2-[(2S,3R,4S,5R)-5-(aminomethyl)-3,4-dihydroxytetrahydrofuran-2-yl]-N-(pyridin-2-ylmethyl)acetamide | C13 H19 N3 O4 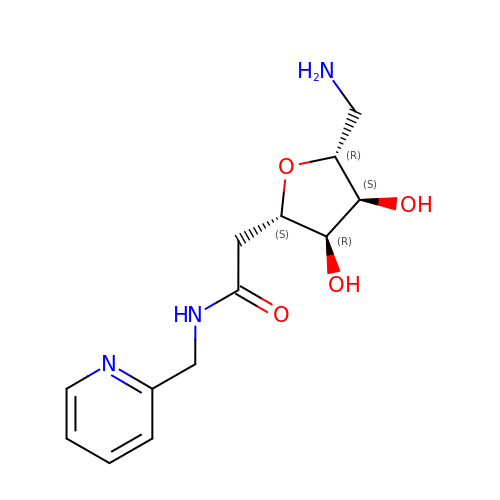| BIGFPMOCLWRIMB-JULQROHOSA-N>[2x]SMGCET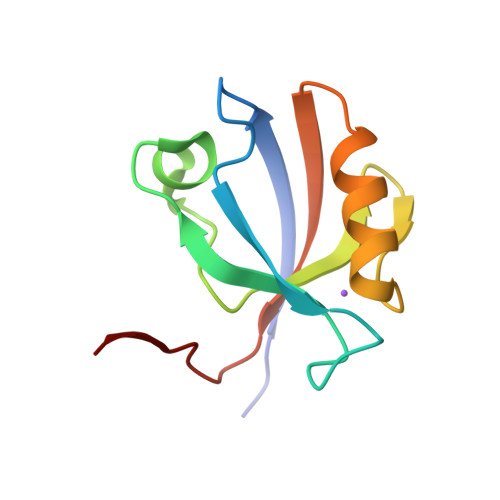TIEISKGRTGLGLSIVGGSDTLLGAIIIHEVYEEGAACKDGRLWAGDQILEVNGIDLRKATHDEAINVLRQTPQRVRLTLYRDEAPYKSTRL Human bestrophin1 (hBest1) is a Ca2+-activated Cl− channel essential for Cl− transport in retinal pigment epithelium (RPE). Although the structure of hBest1 is still unsolved, two Best1 homolog structures, one from bacteria Klebsiella pneumoniae (KpBest) and the other from chicken (cBest1), have been previously reported. Overall, the channel is a pentameric assembly with a single ion-conducting pathway, which varies in diameter along its length and is constrained at two narrow points: a “neck” contributed by three residues (I62/I66/F70 in KpBest and I76/F80/F84 in hBest1/cBest1) on a transmembrane helix, and an “aperture” formed by a single residue (I180 in KpBest1, I205 in hBest1, and V205 in cBest1) on a cytosolic helix. Here, by electrophysiological and structural analyses, we show that the neck and aperture in hBest1 are both indispensable Ca2+-dependent gates, and their dysregulated opening by rationally designed or patient-derived mutations causes Ca2+-independent leak and elevates Ca2+-dependent channel activity.

hBest1 D203A is a patient-derived mutation localized on an intracellular loop adjacent to the aperture. Structural analysis predicted a local alteration by this alanine substitution, as the corresponding residue in KpBest (D179) is involved in a D179–R172 salt bridge formation. Strikingly, the KpBest D179A structure showed a bigger opening at the aperture (radius 1.5 Å) with a slightly twisted I180 possibly caused by disruption of the D179–R172 salt bridge, and conformational changes at all three newly identified neck-controlling residues (P208, Y211, and W252). This suggests a crucial role of this residue (KpBest D179 and hBest1 D203) in the regulation of both the neck and aperture. Notably, the aspartic acid–arginine salt bridge is not present in hBest1 because the residue corresponding to R172 of KpBest1 (R196 in cBest1) is W196 in hBest1. Consistently, hBest1 D203A displayed electrophysiological properties reflecting changes at both gates: first, the Ca2+-dependent Cl− current was bigger than that from WT hBest1, indicating a gain-of-function phenotype; second, Ca2+-independent leak of Cl−, but not of CH3SO3−, was recorded, suggesting an incomplete closure of the aperture (like hBest1 I205T); third, while the relative permeability of CH3SO3−/Cl− was retained, the trans-promotive effect of CH3SO3− was abolished, indicating dysregulated gating at the neck (like hBest1 3A, Y236A/C, and W287F). Taken together, our results suggest that D203 serves as a communication point of the two gates, while hBest1 D203A is a gain-of-function mutation due to enhanced opening of both the neck and aperture.

>[5x]SNAMIIRPEQHWFLRLFDWHGSVLSKIIFRLLLNVLMSIIAIISYQWYEQLGIHLTVAPFSLLGIAIAIFLGFRNSASYSRFVEARNLWGTVLIAERTLVRQLRNILPAEHDAHRRIVSYLVAFSWSLKHQLRKTDPTADLRRLLPEERVTEILASSMPTNRILLLAGNEIGQLREAGKLSAITYGLMDNKLDELAHVLGGCERLATTPVPFAYTLILQRTVYLFCTLLPFALVGDLHYMTPFVSVFISYTFLSWDSLAEELEDPFGTAANDLPLNAMCNTIERNLLDMTGQHPLPE> GSKPHQWQADEEAVRSATCSFSVKY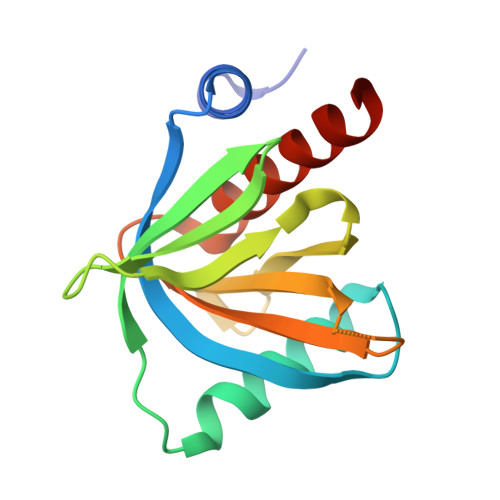LGCVEVFESRGMQVCEEALKVLRQSRRRPVRGLLHVSGDGLRVVDDETKGLIVDQTIEKVSFCAPDRNHERGFSYICRDGTTRRWMCHGFLACKDSGERLSHAVGCAFAVCLERKQ>[4x]SMTVRFGLLGAG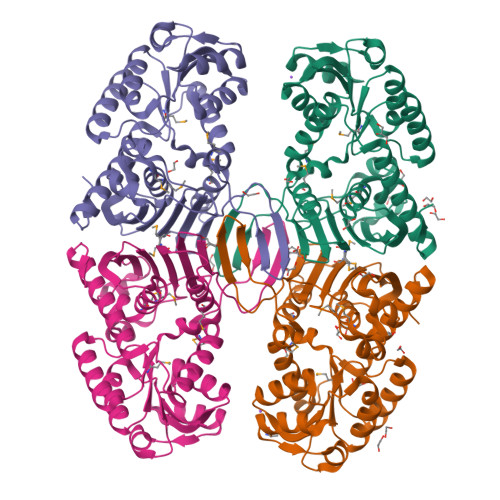RIGKVHAKAVSGNADARLVAVADAFPAAAEAIAGAYGCEVRTIDAIEAAADIDAVVICTPTDTHADLIERFARAGKAIFCEKPIDLDAERVRACLKVVSDTKAKLMVGFNRRFDPHFMAVRKAIDDGRIGEVEMVTITSRDPSAPPVDYIKRSGGIFRDMTIHDFDMARFLLGEEPVSVTATAAVLIDKAIGDAGDYDSVSVILQTASGKQAIISNSRRATYGYDQRIEVHGSKGAVAAENQRPVSIEIATGDGYTRPPLHDFFMTRYTEAYANEIESFIAAIEKGAEIAPSGNDGLAALALADAAVRSVAEKRQISIA>[8x]MIPDDEFIKNPSVPGPTAMEVRCLIMCLAEPGKNDVAVDVGCG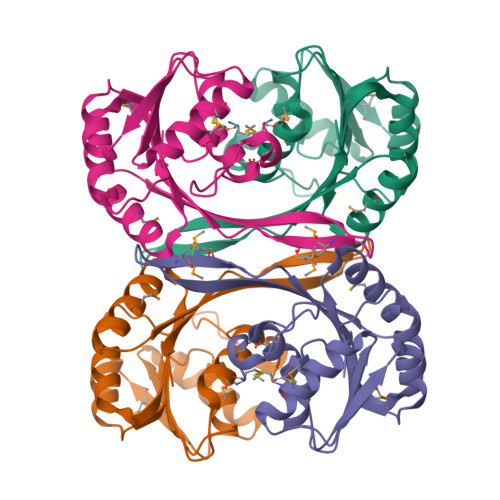TGGVTLELAGRVRRVYAIDRNPEAISTTEMNLQRHGLGDNVTLMEGDAPEALCKIPDIDIAVVGGSGGELQEILRIIKDKLKPGGRIIVTAILLETKFEAMECLRDLGFDVNITELNIARGRALDRGTMMVSRNPVALIYTGVSHENKD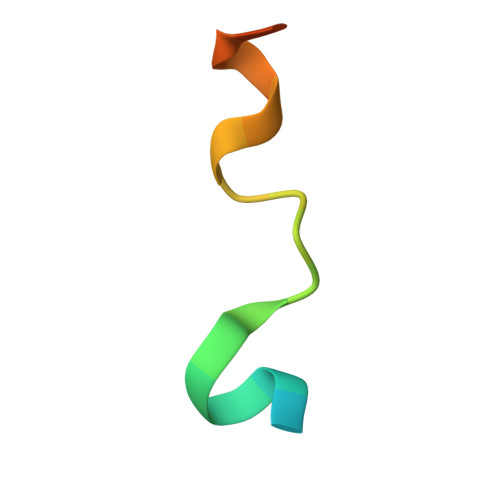> GSHMFFEIFGTGEEYRYVLESDP> MDAAEVEFLAEKELVTIIPNFSLDKIYLIGGDLGPFNPGLPVEVPLWLAINLKQRQKCRLLPPEWMDVEKLEKMRDHERKEETFTPMPSPYYMELTKLLLNH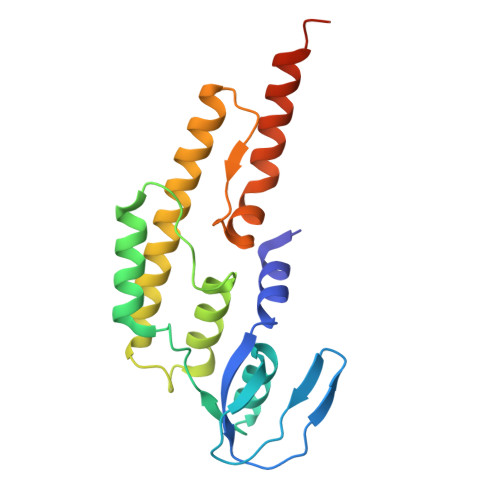ASDNIPKADEIRTLVKDMWDTRIAKLRVSADSFVRQQEAHAKLDNLTLMEINTSGTFLTQALNHMYKLRTNLQPLESTQSQDF>[2x]MPKPINVRVTTMDAELEFAIQPNTTGKQLFDQVVKTIGLREVWYFGLHYVDNKGFPTW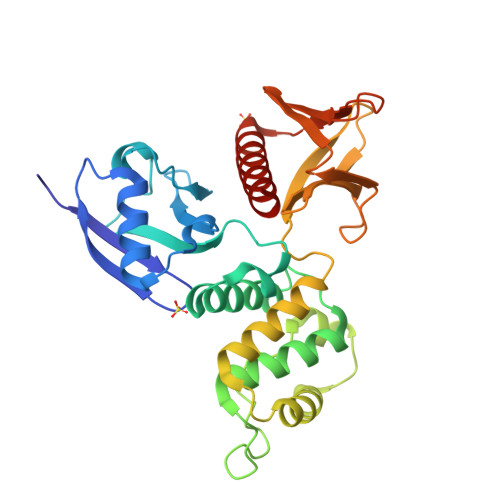LKLDKKVSAQEVRKENPLQFKFRAKFYPEDVAEELIQDITQKLFFLQVKEGILSDEIYCPPETAVLLGSYAVQAKFGDYNKEVHKSGYLSSERLIPQRVMDQHKLTRDQWEDRIQVWHAEHRGMLKDNAMLEYLKIAQDLEMYGINYFEIKNKKGTDLWLGVDALGLNIYEKDDKLTPKIGFPWSEIRNISFNDKKFVIKPIDKKAPDFVFYAPRLRINKRILQLCMGNHELYMRRRK N-(4-{2-[(6S)-2-amino-4-oxo-1,4,5,6,7,8-hexahydropyrido[2,3-d]pyrimidin-6-yl]ethyl}benzoyl)-L-glutamic acid | C21 H25 N5 O6 | 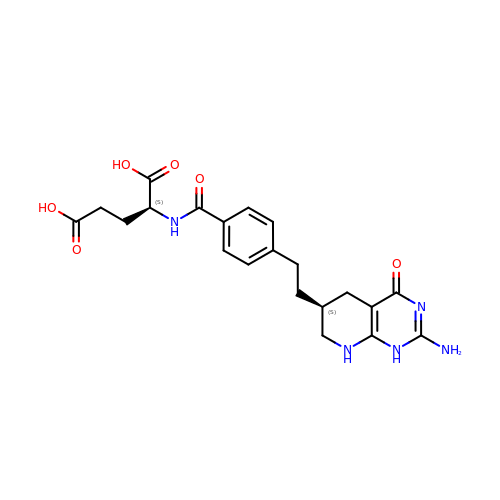ZUQBAQVRAURMCL-WFASDCNBSA-N> GSHMTQFAFVFPGQGSQTVGMLADMAASYPIVEETFAEASAALGYDLWALTQQGPAEELNKTWQTQPALLTASVALYRVWQQQGGKAPAMMAGHCLGEYSALVCAGVIDFADAVRLVEMRGKFMQEAVPEGTGAMAAIIGLDDASIAKACEEAAEGQVVSPVNFNSPGQV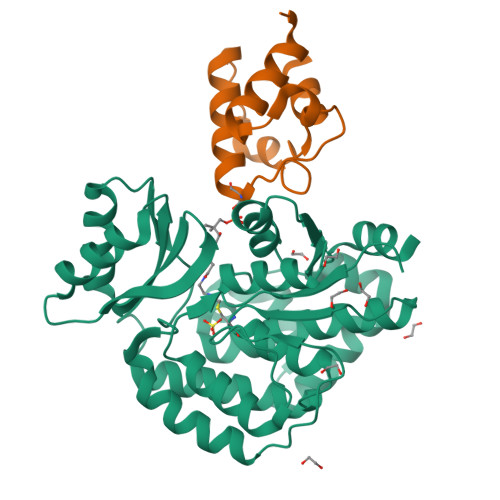VIAGHKEAVERAGAACKAAGAKRALPLPVSVPSHCALMKPAADKLAVELAKITFNAPTVPVVNNVDVKCETNGDAIRDALVRQLYNPVQWTKSVEYMAAQGVEHLYEVGPGKVLTGLTKRIVDTLTASALNEPSAMAAALEL;> MSTIEERVKKIIGEQLGVKQEEVTNNASFVEDLGADSLDTVELVMALEEEFDTEIPDEEAEKITTVQAAIDYINGHQASHHHHHH>[4x]SNAERLAAWTRLPWEGLRYSYNR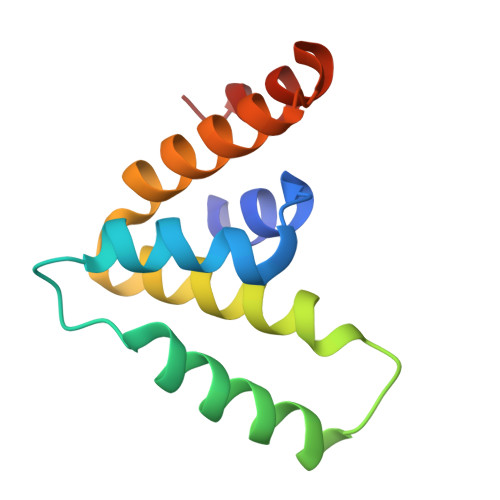ERRGTAARSCPQLEADVALKAETQPSEIPLERQLILEACREAERFGFLHELSIAIVEMERLNKRPEAEVEEIAKLWQ> TSITA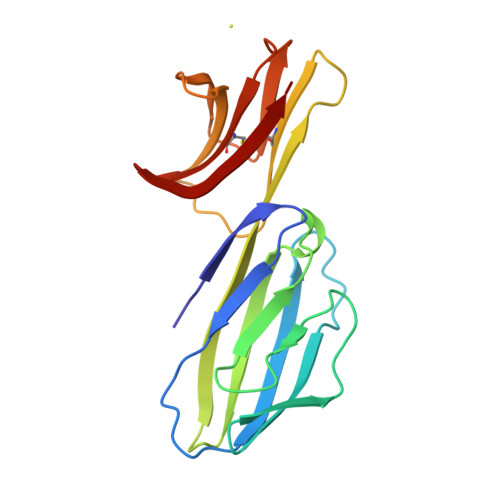YKSEGESAEFSFPLNLGEESLQGELRWKAEKAPSSQSWITFSLKNQKVSVQKSTSNPKFQLSETLPLTLQIPQVSLQFAGSGNLTLTLDRGILYQEVNLVVMKVTQPDSNTLTCEVMGPTSPKMRLILKQENQEARVSRQEKVIQVQAPEAGVWQCLLSEGEEVKMDSKIQV>HHHHHHENLYFQSMAVSPSPLRIFTAGGTIDQDYRLEENGLVVGDPFVAEVLKTARLAGAVSIVALSRKDSLDFTEADREAIGRAVGQAVEDHILLTHGTDTMVETARYLGGLPELAGKTVVLSGAMVPGRVGGSDAAFNIGFACAAALMLAPGVYIAMHGKVFDPAKTRKNRGLGRFEPIDDQE[2x]

L‐Asparaginases (ASNases) catalyze the hydrolysis of L‐Asn to L‐Asp and ammonia. In contrast, the chain of ASNase from Rhodospirillum rubrum, reported here and referred to as RrA, consists of only 172 amino acid residues. RrA is homologous to the N‐terminal domain of typical bacterial class 1 ASNases and exhibits millimolar affinity for L‐Asn. Crystal structures of the wild‐type RrA, both with and without bound L‐Asp, as well as structures of several RrA mutants, reveal topologically unique tetramers.

A distinctive feature of RrA is the presence of Lys19 within the lining of the substrate‐binding site. We probed the importance of this residue by mutating it to L‐Ala, L‐Glu, and L‐Gln. Crystals of RrA(K19Q) were grown both in the absence and presence of L‐Asp in the crystallization buffer. However, aspartate could not be modeled in either structure, although some density found in the active sites appeared to represent molecules other than water. Gln19 interacts indirectly with the OH of Tyr21 of an adjacent protomer through a water molecule. There were no disordered regions in the main chain of any protomer, aside from some N‐ and C‐terminal residues. The kinetic data, even when reduced to approximate turnover numbers, demonstrate that Lys19 plays an important role during catalysis and its mutation reduces the rate of catalysis by two or more orders of magnitude.> SNAIRPTIGQQMETGDQRFGDLVFRQLAPNVWQHTSYLDMPGFGAVASNGLIVRDGGRVLVVDTAWTDDQTAQILNWIKQEINLPVALAVVTHFHQDKMGGMDALHAAGIATYANALSNQLAPQEGMVAAQHSLTFAANGWVEPATAPNFGPLKVFYPGPGHT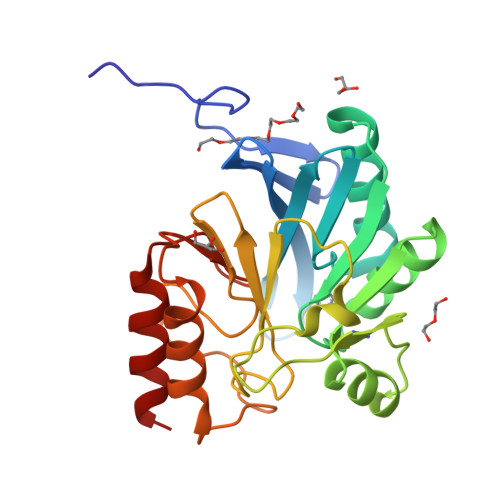SDNITVGIDGTDIAFGGCLIKDSKAKSLGNLGDADTEHYAASARAFGAAFPKASMIVMSHSAPDSRAAITHTARMADKLR> MDN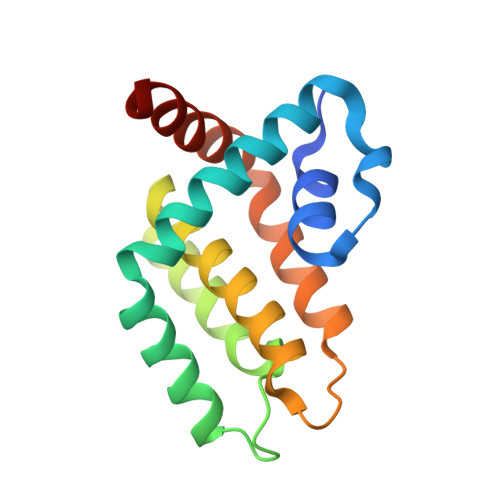CNYNIEKVLNVYLRDLRIESLNNNELEILIMIRECCEVIKKDYKTEFNEICNFILQNNVKSCYDINDVKNIIIETINSDFRPSVILASISLLSIIIKKKKDENNEVVDDDLALNELINKFSSYQKDIISFVEKNKKKNKQND> MNNVVIRHHCKPLTIAQQYRALKAGGPYERLRIIHHDRTLLWEGWLQPSLFSRRYKVAVRYSLGTPPICVVTEPDLFALAGTRAIPHLYPADKHIPGARLCLF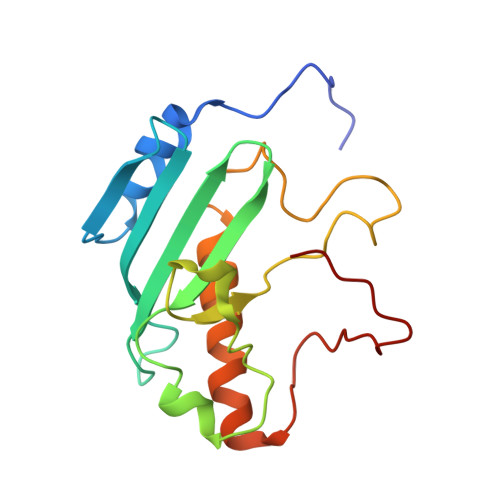LPRSQADDGLSEWRAQLKISDTLIPWASLWLFYFEQWLHTGHWEGGGKHPRPSEVKNER> MELKHSISDYTEAEFLQLVTTICNADTSSEEEL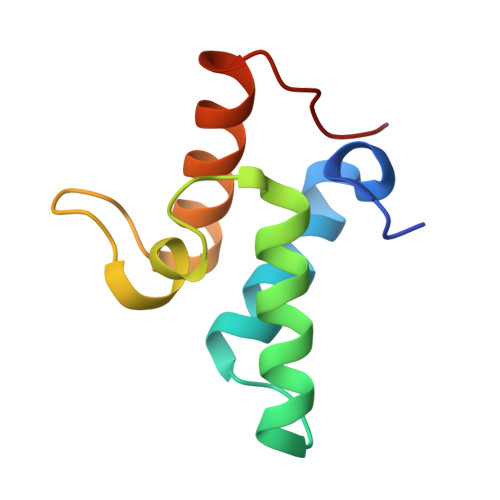VKLVTHFEEMTEHPSGSALIYYPKEGDDDSPSGIVNTVKQWRAANGKSGFKQG> MHHHHHHNTFIFPATFMWGTSTSSYQIEGGTDEGGRTPSIWDTFCQIPGKVIGGDCGDVACDHFHHFKEDVQLMKQLGFLHYRFSVAWPRIMPAAGIINEEGLLFYEHLLDEIELAGLIPMLTLYHWDLPQWIEDEGGWTQRETIQHFKTYASVIMDRFGERINWWN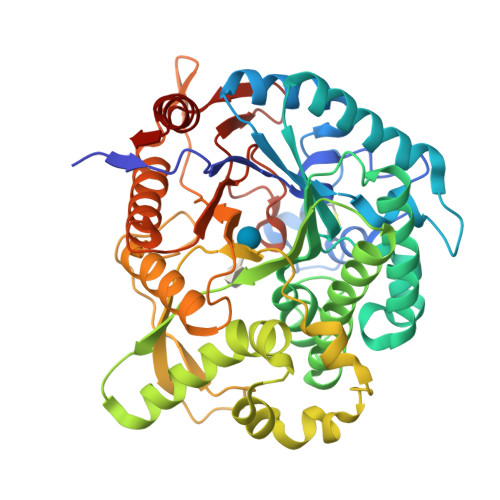TINEPYCASILGYGTGEHAPGHENWREAFTAAHHILMCHGIASNLHKEKGLTGKIGITLNMEHVDAASERPEDVAAAIRRDGFINRWFAEPLFNGKYPEDMVEWYGTYLNGLDFVQPGDMELIQQPGDFLGINYYTRSIIRSTNDASLLQVEQVHMEEPVTDMGWEIHPESFYKLLTRIEKDFSKGLPILITENGAAMRDELVNGQIEDTGRQRYIEEHLKACHRFIEEGGQLKGYFVWSFLDNFEWAWGYSKRFGIVHINYETQERTPKQSALWFKQMMAKNGF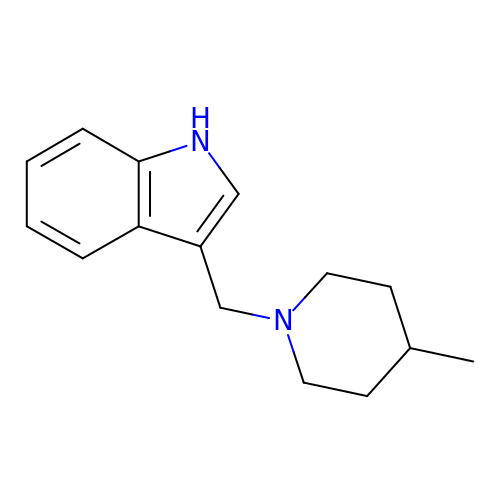3-[(4-methylpiperidin-1-yl)methyl]-1H-indole | C15 H20 N2 | DGCGMYNLCDVYMB-UHFFFAOYSA-N>[6x]STFVAKDGTQIYFKDWGSGKPVLF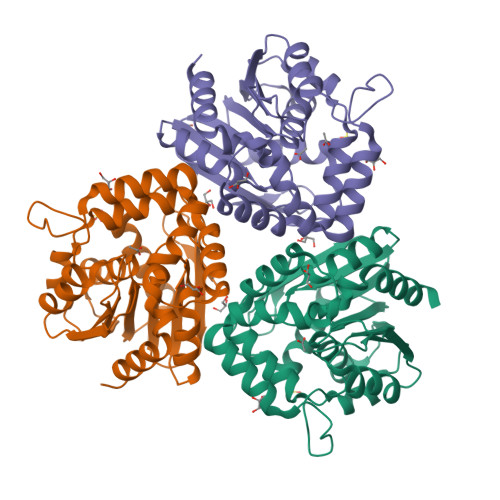SHGWPLDADMWEYQMEYLSSRGYRTIAFDRRGFGRSDQPWTGNDYDTFADDIAQLIEHLDLKEVTLVGFSMGGGDVARYIARHGSARVAGLVLLGAVTPLFGQKPDYPQGVPLDVFARFKTELLKDRAQFISDFNAPFYGINKGQVVSQGVQTQTLQIALLASLKATVDCVTAFAETDFRPDMAKIDVPTLVIHGDGDQIVPFETTGKVAAELIKGAELKVYKDAPHGFAVTHAQQLNEDLLAFLKR> MRRKVKN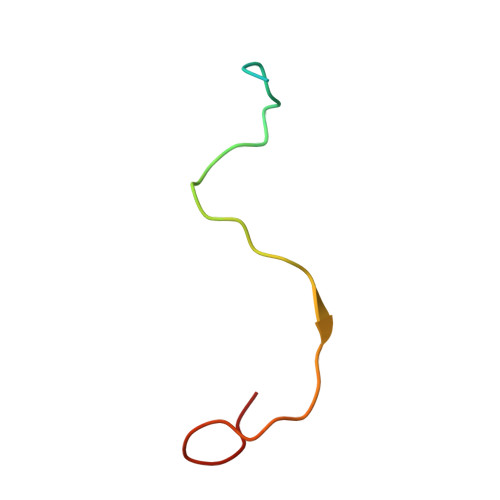TKRHQWRLTHSARSIKRANIMPSNPRGGRRF> RQPEVRGGDTLNVFLAYVPEDAKAMMTTPFEAYLVNDSNYYLYYTYLSAEGKAWNNRSHGLVEPNTKLLLEEFTKD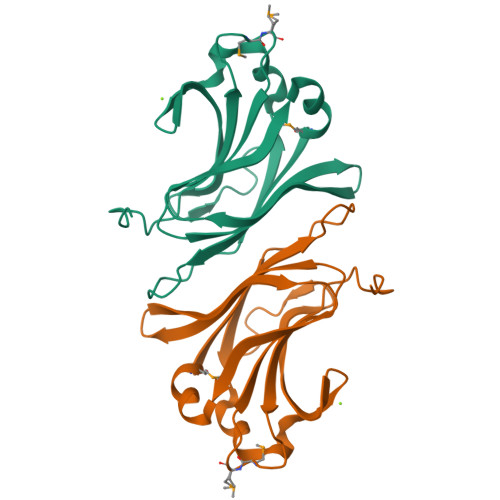VLNEMERVAVQLIAFKDGKPAAIKPAVSVELRIDTVKFYKLHTFSASDFFEEPALIYDIVKDDVPAKQVYV> QASQSIDQLIKRKGKLYFGTATDRGLLQREKNAAIIQADLGQVTPENSMKWQSLENNQGQLNWGDADYLVNFAQQNGKSIRGHTLIWHSQLPAWVNNINNADTLRQVIRTHVSTVVGRYKGKIRAWDVVNEIFNEDGTLRSSVFSRLLGEEFVSIAFRAARDADPSARLYINDYNLDR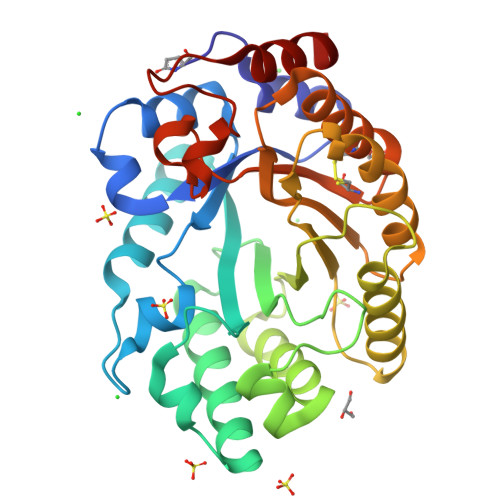ANYGKVNGLKTYVSKWISQGVPIDGIGSQSHLSGGGGSGTLGALQQLATVPVTELAITELDIQGAPTTDYTQVVQACLSVSKCVGITVWGISDKDSWRASTNPLLFDANFNPKPAYNSIVGILQ>MEWDSGSDLSADDASSLADDEEGGLFPGGGPIPYPVGNLLHTAP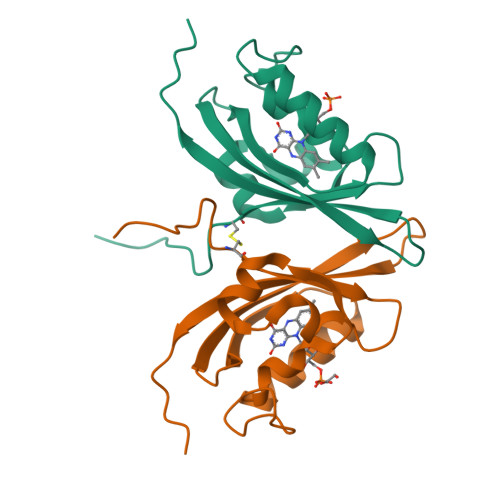CAFVVTDAVEPDQPIIYVNTVFEMVTGYRAEEVLGRNCRFLQCRGPFAKRRHPLVDSMVVSEIRKCIDEGIEFQGELLNFRKDGSPLMNRLRLTPIYGDDDTITHIIGIQFFIETDIDLGPVLGSSTKEKSIDGIYSALAAGERNV[7x]>SSPITGLVYDQRMMLHHNMWDSHHPELPQRISRIFSRHEELRLLSRCHRIPARLATEEELALCHSSKHISIIKSSEHMKPRDLNRLGDEYNSIFISNESYTCALLAAGSCFNSAQAILTGQVRNAVAIVRPPGHHAEKDTACGFCFFNTAALTARYAQSITRESLRVLIVDWDVHHGNGTQHIFEEDDSVLYISLHRYEDGAFFPNSEDANYDKVGLGKGRGYNVNIPWNGGKMGDPEYMAAFHHLVMPIAREFAPELVLVSAGFDAARGDPLGGFQVTPEGYAHLTHQLMSLAAG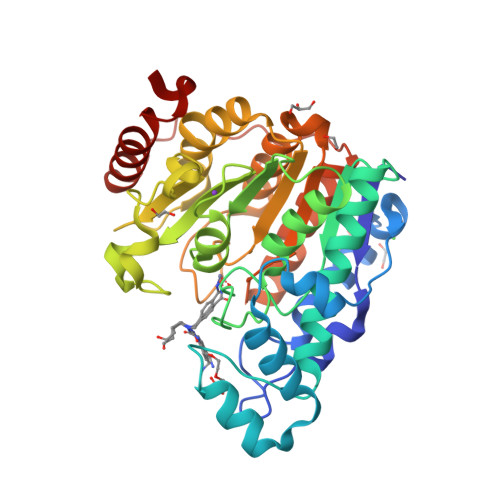RVLIILEGGYNLTSISESMSMCTSMLLGDSPPSLDHLTPLKTSATVSINNVLRAHAPFWSSLR[2x]Using electron cryo-microscopy (cryo-EM) and single particle analysis, we determined the organization of the tail proximal extremity of siphophage T5 that possesses a long flexible tail and solved the structure of its tail terminator protein p142 (TrP142). In siphophages, functional tails are produced after capping of the tail tube by the tail terminator proteins (TrP), of which siphophage λ gpU is the prototype. TrPp142 is resolved as a hexameric ring, interacting with the last tail tube protein TTPpb6 ring. TrPp142 is a 161-residues protein, mainly formed by a four-strand antiparallel β-sheet that lines the lumen of the tube, flanked by two α-helices, and a short loop between β-strands 1 and 2.

T5 tails, purified from a capsid defective mutant, were produced, vitrified for cryo-EM characterization, and imaged for the data collection on a high-end electron microscope. Image analysis yielded a map of T5 tail proximal extremity, containing a trimeric ring of the tail TTPpb6, on top of which sits a hexameric ring formed by the TrPp142. The estimated resolution of this map is 3.9 Å, which allowed us to build pseudo-atomic models for both TrPp142 hexamer and a TTPpb6 trimer. The interaction between the hexameric TrPp142 ring and the trimeric TTPpb6 ring under it is ensured by the tip of loop 63–67, which inserts in two similar pockets resulting in the domain duplication of TTPpb6 (14) and is mostly mediated by electrostatic interactions. As the TrPp142 hexameric ring sits on top of a TTPpb6 trimeric ring, it exhibits a C3/pseudo-C6 symmetry and two consecutive TrPp142 monomers are not strictly identical. However, TTPpb6 also exhibits a C3/pseudo-C6 symmetry as it results in domain duplication (excluding its Ig-like domain); thus, the two consecutive TrPp142 monomers are almost superimposable (rmsd = 1.02 Å over 156 residues). The unsharpened cryo-EM map of the T5 tail proximal extremity shows a 25 Å diameter large, cylindrical, and ill-defined density filling the tail tube lumen to the top of TrPp142, which disappears from the map after interaction with FhuA. This density most probably belongs to the N-terminus of the Tape Measure Protein pb2 (TMPpb2), which fills the entire tail tube in native phages and purified tails. In the lumen of the tail tube before interaction with the receptor, densities of much lower resolution are present, which we attribute to TMPpb2. Thus, there is no unassigned density in this proximal extremity map of the tail that could account for TCPp143.

>MDHRTSIAQAMVDRISKQMDGSQPDEYFNNLYGNVSRQTYKFEEIREFPYVAVHIGTETGQYLPSGQQWMFLELPILVYDKEKTDIQEQLEKLVADIKTVIDTGGNLEYTVSKPNGSTFPCEATDMIITSVSTDEGLLAPYGLAEINVTVRYQPPRRSLRR[6x];>MSLQLLRNTRIFVSTVKTGHNKTNTQEILVQDDISWGQDSNSTDITVNEAGPRPTRGSKRFNDSLNAAEWSFSTYILPYKDKNTSKQIVPDYMLWHALSSGRAINLEGTTGAHNNATNFMVNFKDNSYHELAMLHIYILTDKTWSYIDSCQINQAEVNVDIEDIGRVTWSGNGNQLIPLDEQPFDPDQIGIDDETYMTIQGSYIKNKLTILKIKDMDTNKSYDIPITGGTFTINNNITYLTPNVMSRVTIPIGSFTGAFELTGSLTAYLNDKSLGSMELYKDLIKTLKVVNRFEIALVLGGEYDDERPAAILVAKQAHVNIPTIETDDVLGTSVEFKAIPSDLDAGDEGYLGFSSKYTRTTINNLIVNGDGATDAVTAITVKSAGNVTTLNRSATLQMSVEVTPSSARNKEVTWAITAGDAATINATGLLRADASKTGAVTVEATAKDGSGVKGTKVITVTAGG[3x]> MAVPSSKEELIKAINSNFSLLNKKLESITPQLAFEPLLEGHAKGTTISVAN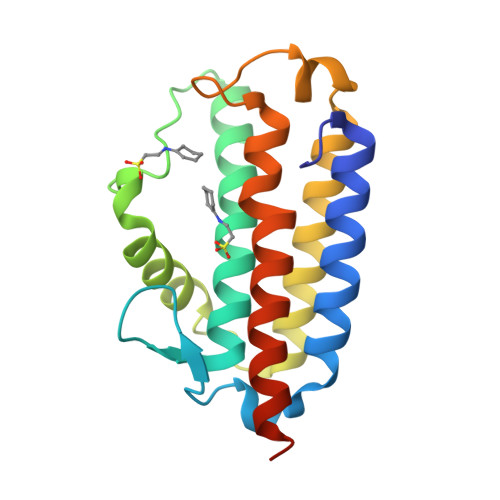LVSYLIGWGELVLHWHDQEAKGKTIIFPEEGFKWNELGRLAQKFYRDYEDITEYEVLLARLKENKQQLVALIERFSNDELYGKPWYNKWTRGRMIQFNTASPYKNASGRLNKLQKCLAELEHHHHHH> EPVET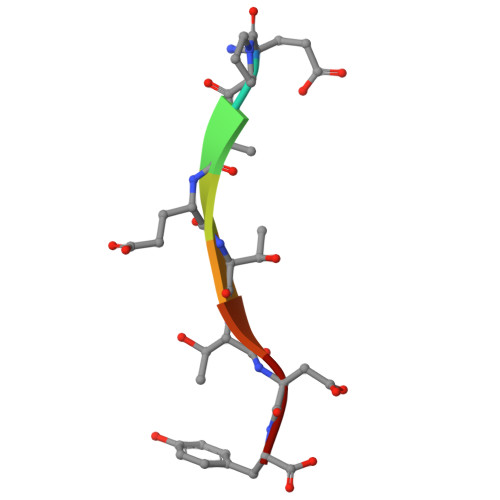TDY> MSAIKPDMKIKLRMEGNVNGHHFVIDGDGTGKPFEGKQSMDLEVKEGGPLPFAFDILTTAFAYGNRVFAKYPDNIQDYFKQSFPKGYSWERSLTFEDGGICNARNDITMEGDTFYNKVRFYGTNFPANGPVMQKKTLKWEPSTEKMYVRDGVLTGDVETALLLEGNAHYRCDFRTTYKAKEKGVKLPGAHFVDHCIEILSHDKDYNKVKLYEHAVAHSGLPN;> MSAIKPDMKIKLRMEGNVNGHHFVIDGDGTGKPFEGKQSMDLEVKEGGPLPFAFDILTTAFXNRVFAKYPDNIQDYFKQSFPKGYSWERSLTFEDGGICNARNDITMEGDTFYNKVRFYGTNFPANGPVMQKKTLKWEPSTEKMYVRDGVLTGDVETALLLEGNAHYRCDFRTTYKAKEKGVKLPGAHFVDHCIEILSHDKDYNKVKLYEHAVAHSGLPN

The system studied was a reversibly switchable fluorescent protein (rsFP) which is a representative of a class of proteins that undergo a reversible photolysis reaction from a highly fluorescent “on” state to a weakly fluorescence “off” state. The specific rsFP used, rsKiiro, is a mutant of Skylan-NS33 specifically developed for ultrafast time-resolved crystallographic studies due to its ability to form crystals that diffract to high resolution (∼1.1 Å for single-crystal cryo-MX), high photoswitching quantum yield (∼18% Trans-to-Cis in the crystal), and high protein expression yields. Structurally, rsKiiro is similar to green fluorescent protein (GFP) with an 11-stranded β-barrel surrounding an α helix. The chromophore of rsKiiro is formed from the Ala-Tyr-Gly tripeptide at residue numbers 62–64 in the α helix.

In this study, we probed the light-induced reverse reaction, from the Trans to Cis chromophore conformation, initiated with 2 ms 405 nm pulses at a range of optical flash energy densities (0.1–6.7 mJ/mm2) after the initial Cis-to-Trans photoconversion had been driven to completion using ∼13 mW/mm2 of 473 nm CW illumination. A total of 435,200 images were obtained across 6 laser energy densities at 405 nm of 0, 0.1, 0.53, 1.78, 6.74, and 14.43 mJ/mm2. From these images, 79,976 single-crystal indexed diffraction patterns were obtained and merged into 6 data sets for each corresponding laser energy density. Data below a value of 0.5 in Fourier shell correlation were discarded, leading to a uniform limit of 1.7 Å being applied to all data sets. The initial examination of the chromophore-omitted maps clearly shows increasing occupancy of the Cis state at higher energy densities.>MRLELPVIPLRNTVILPHTTTPVDVGRAKSKRAVEEAMGADRLIFLVAQRDPEVDDPAPDDLYTWGVQAVVKQAMRLPDGTLQVMVEARARAQVTDYIPGPYLRARGEVFSEIFPIDEAVVRVLVEELKEAFEKYVANHKSLRLDRYQLEAVKGTSDPAMLADTIAYHATWTVAEKQEILELTDLEARLKKVLGLLSRDLERFELDKRVAQRVKEQMDTNQREYYLREQMKAIQKELGGEDGLSDLEALRKKIEEVGMPEAVKTKALKELDRLERMQQGSPEATVARTYLDWLTEVPWSKADPEVLDINHTRQVLDEDHYGLKDVKERILEYLAVRQLTQGLDVRNKAPILVLVGPPGVGKTSLGRSIARSMNRKFHRISLGGVRDEAEIRGHRRTYIGAMPGKLIHAMKQVGVINPVILLDEIDKMSSDWRGDPASAMLEVLDPEQNNTFTDHYLDVPYDLSKVFFITTANTLQTIPRPLLDRMEVIEIPGYTNMEKQAIARQYLWPKQVRESGMEGRIEVTDAAILRVISEYTREAGVRGLERELGKIARKGAKFWLEGAWEGLRTIDASDIPTYLGIPRYRPDKAETEPQVGTAQGLAWTPVGGTLLTIEVAAVPGSGKLSLTGQLGEVMKESAQAALTYLRAHTQDYGLPEDFYNKVDLH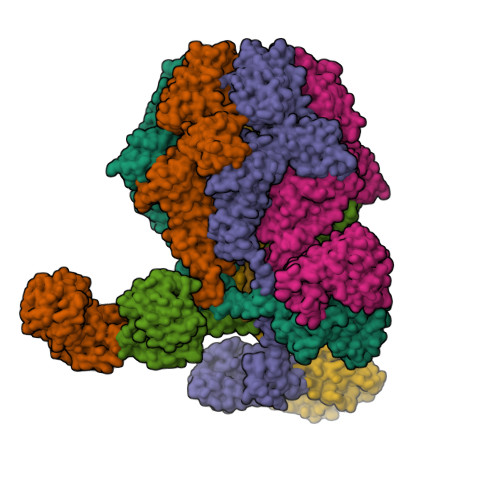VHVPDGATPKDGPSAGITMATAIASALSRRPARMDIAMTGEVSLRGKVMPIGGVKEKLLAAHQAGIHKIVLPKDNEAQLEELPKEVLEGLEIKLVEDVGEVLEYLLLPEPTMPPVVQPSDNRQQPGAGAKLAAALEHHHHHH[6x]>TVDVGPDSVKSACIEVDIQQTFFDKTWPRPIDVSKADGIIYPQGRTYSNITITYQGLFPYQGDHGDMYVYSAGHATGTTPQKLFVANYSQDVKQFANGFVVRIGAAANSTGTVIISPSTSATIRKIYPAFMLGSSVGNFSDGKMGRFFNHTLVLLPDGCGTLLRAFYCILEPRSGNHCPAGNSYTSFATYHTPATDCSDGNYNRNASLNSFKEYFNLRNCTFMYTYNITEDEILEWFGITQTAQGVHLFSSRYVDLYGGNMFQFATLPVYDTIKYY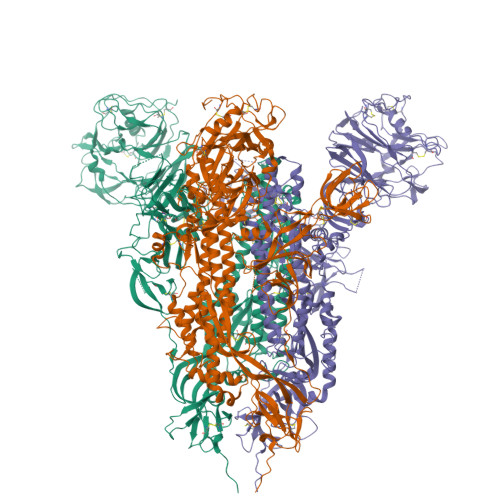SIIPHSIRSIQSDRKAWAAFYVYKLQPLTFLLDFSVDGYIRRAIDCGFNDLSQLHCSYESFDVESGVYSVSSFEAKPSGSVVEQAEGVECDFSPLLSGTPPQVYNFKRLVFTNCNYNLTKLLSLFSVNDFTCSQISPAAIASNCYSSLILDYFSYPLSMKSDLSVSSAGPISQFNYKQSFSNPTCLILATVPHNLTTITKPLKYSYINKCSRFLSDDRTEVPQLVNANQYSPCVSIVPSTVWEDGDYYRKQLSPLEGGGWLVASGSTVAMTEQLQMGFGITVQYGTDTNSVCPKLEFANDTKIASQLGNCVEYSLYGVSGRGVFQNCTAVGVRQQRFVYDAYQNLVGYYSDDGNYYCLRACVSVPVSVIYDKETKTHATLFGSVACEHISSTMSQYSRSTRSMLKRRDSTYGPLQTPVGCVLGLVNSSLFVEDCKLPLGQSLCALPDTPSTLTPRSVRSVPGEMRLASIAFNHPIQVDQLNSSYFKLSIPTNFSFGVTQEYIQTTIQKVTVDCKQYVCNGFQKCEQLLREYGQFCSKINQALHGANLRQDDSVRNLFASVKSSQSSPIIPGFGGDFNLTLLEPVSISTGSRSARSAIEDLLFDKVTIADPGYMQGYDDCMQQGPASARDLICAQYVAGYKVLPPLMDVNMEAAYTSSLLGSIAGVGWTAGLSSFAAIPFAQSIFYRLNGVGITQQVLSENQKLIANKFNQALGAMQTGFTTTNEAFQKVQDAVNNNAQALSKLASELSNTFGAISASIGDIIQRLDPPEQDAQIDRLINGRLTTLNAFVAQQLVRSESAALSAQLAKDKVNECVKAQSKRSGFCGQGTHIVSFVVNAPNGLYFMHVGYYPSNHIEVVSAYGLCDAANPTNCIAPVNGYFIKTNNTRIVDEWSYTGSSFYAPEPITSLNTKYVAPQVTYQNISTNLPPPLLGNSTGI[3x]4-[5-amino-4-(3'-amino[1,1'-biphenyl]-3-yl)-1H-pyrazol-3-yl]phenol 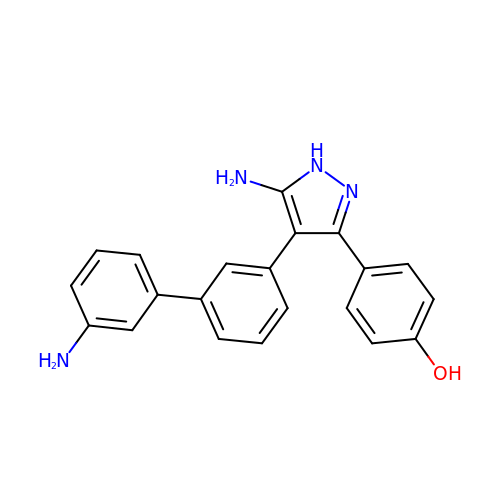| C21 H18 N4 O | BUIBXSQEEVVBFQ-UHFFFAOYSA-N ethyl 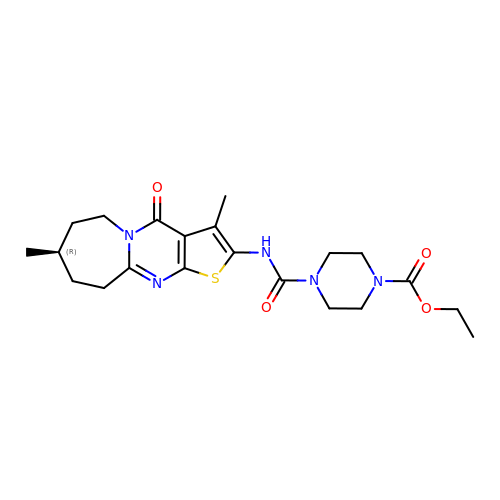4-[(8R)-3,8-dimethyl-4-oxo-4,6,7,8,9,10-hexahydrothieno[2',3':4,5]pyrimido[1,2-a]azepin-2-yl]carbamoylpiperazine-1-carboxylate | C21 H29 N5 O4 S | XBHQVTSPEFNYKC-CYBMUJFWSA-N>MGQGPELHLASQFVNEACRALVFGGCVEKSSVSRNPEVPFESSAYRISASARGKELRLILSPLPGAQPQQEPLALVFRFGMSGSFQLVPREELPRHAHLRFYTAPPGPRLALCFVDIRRFGRWDLGGKWQPGRGPCVLQEYQQFRENVLRNLADKAFDRPICEALLDQRFFNGIGNYLRAEILYRLKIPPFEKARSVLEALQQHRPSPELTLSQKIRTKLQNPDLLELCHSVPKEVVQLGGKGYGSESGEEDFAAFRAWLRCYGMPGMSSLQDRHGRTIWFQGDPGPLAPKGRKS[3x]

Human endonuclease VIII-like 1 (hNEIL1) is a bifunctional DNA glycosylase of the Fpg/Nei family, which catalyzes the removal of damaged bases and subsequent incision of the newly generated abasic sites. Unlike traditional enzymes which are commonly referred to as highly specific biocatalysts, one special feature for hNEIL1 is its unique capability to recognize a wide range of substrates, including formamidopyrimidines, hydantoin lesions, oxidized, and dihydro-modified pyrimidine bases, derived from all four canonical bases. Here, by integrating structural, computational, and biochemical investigations, we show that hNEIL1 uses a triage mechanism to achieve broad specificity and reduce futile repair of normal bases. This mechanism involves two mutually competing interaction states: an activated state that commits catalysis and BER, and a quarantine state that temporarily separates and prevents the flipped base from catalysis via auto-inhibition.

While we also crystallized the complex structures for more lesions in this study, we were unable to obtain intact substrates in the active site of hNEIL1, presumably due to the residual glycosylase activity. Hence, we introduced an extra E3Q mutation to the truncated hNEIL1(C∆95 P2G) (see the “Methods” section) and succeeded in the determination of complex structures containing 5-hydroxyuracil (5-OHU), spiroiminodihydantoin 1 (Sp1), (S)-guanidinohydentoin (Gh), dihydrothymine (DHT) and dihydrouracil (DHU), respectively. Despite the very different chemical structures of these substrates, they are recognized similarly by hNEIL1. The damaged bases are fully extruded from the DNA helix and inserted into a relatively loose binding pocket, which allows the accommodation of substrates with varying sizes and shapes. One edge of the flipped base points towards the protein and forms close contact with the side chain of K242. Noteworthy, across all these structures, we observed an unusually short distance (~3.0 Å) between an outwards heterocyclic nitrogen atom of the nucleobases and the terminal nitrogen atom of residue 242. Based on the similar overall conformation and detailed atomic interactions, we conclude that such a tautomerization-dependent mechanism may be a general strategy for hNEIL1 to recognize not only Tg but also 5-OHU, Sp1, Gh, DHT, and DHU. Moreover, it is expected that the bases with less solvent interactions (e.g. DHU) would favor the formation of a stable quarantine state compared with the hydrophilic bases (Sp1, 5-OHU, Gh, and Tg).> MSTGFSFGSGTLGSTTVAAGGTSTGGVFSFGTGASSNPSVGLNFGNLGSTSTPATTSAPSSGFGTGLFGSKPATGFTLGGTNTGIATTITTGLTLGTPATTSAATTGFSLGFNKPAASATPFALPITSTSASGLTLSSALTSTPAASTGFTLNNLGGTTATTTTASTGLSLGGALAGLGGSLFQSTNTGTSGLGQNALGLTLGTTAATSTAGNEGLGGIDFSSSSDKKSDKTGTRPEDSKALKDENLPPVICQDVENLQKFVKEQKQVQEEISRMSSKAMLKVQEDIKALKQLLSLAANGIQRNTLNIDKLKIETAQELKNAEIALRTQKTPPGLQHEYAAPADYFRILVQQFEVQLQQYRQQIEELENHLATQANNSHITPQDLSMAMQKIYQTFVALAAQLQSIHENVKVLKEQYLGYRKMFLGDAVDVFETRRAEAKKWQNTPRVTTGPTPFSTMPNAAAVAMAATLTQQQQPATGPQPSLGVSFGTPFGSGIGTGLQSSGLGSSNLGGFGTSSGFGCSTTGASTFGFGTTNKPSGSLSAGFGSSSTSGFNFSN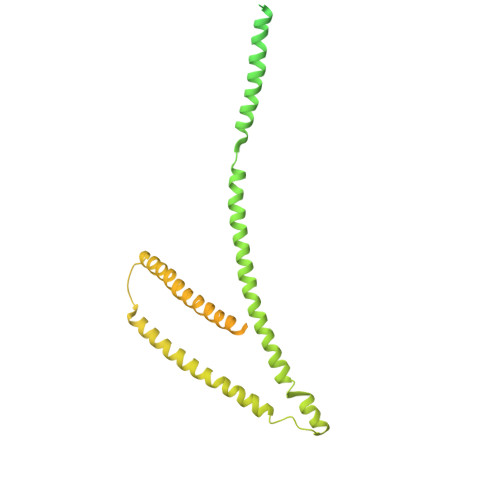PGITASAGLTFGVSNPASAGFGTGGQLLQLKKPPAGNKRGKR>MQQGQMAYDRAITVFSPDGRLFQVEYAREAVKKGSTALGMKFANGVLLISDKKVRSRLIEQNSIEKIQLIDDYVAAVTSGLVADARVLVDFARISAQQEKVTYGSLVNIENLVKRVADQMQQYTQYGGVRPYGVSLIFAGIDQIGPRLFDCDPAGTINEYKATAIGSGKDAVVSFLEREYKENLPEKEAVTLGIKALKSSLEEGEELKAPEIASITVGNKYRIYDQEEVKKFL[7x];>[7x]MNQTLETGTTTVGITLKDAVIMATERRVTMENFIMHKNGKKLFQIDTYTGMTIAGLVGDAQ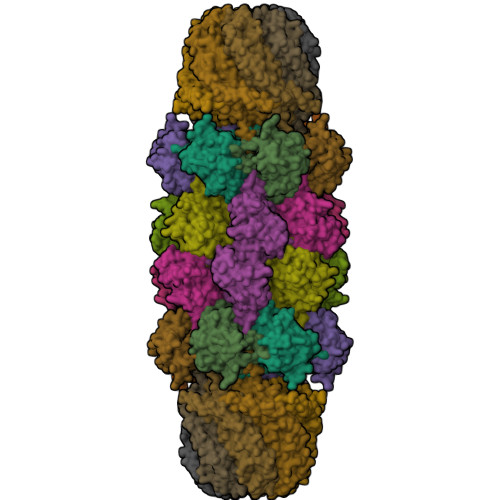VLVRYMKAELELYRLQRRVNMPIEAVATLLSNMLNQVKYMPYMVQLLVGGIDTAPHVFSIDAAGGSVEDIYASTGSGSPFVYGVLESQYSEKMTVDEGVDLVIRAISAAKQRDSASGGMIDVAVITRKDGYVQLPTDQIESRIRKLGLILHHHHHH;>MAHHHHHHPPKRAALIQNLRDSYTETSSFAVIEEWAAGTLQEIEGIAKAAVEAHATIRNSTYGRAQAEKSPEQLLGVLQRYQDLCHNVYCQAETIRTVIAIRIPEHKEADNLGVAVQHAVLKVIDELEIKTLGSGEKSGSGGAPTPIGMYALREYLSARSTVEDKLLGSVDAESGKTKGGSQSPSLLLELRQIDADFMLKVELATTHLSTMVRAVINAYLLNWKKLIQPRGGHLDVLYR[7x]>[5x]QELGNANFENFIGATEGFSEIAYQFTSHILTLGYAVMLAGLLYFILTIKNVDKKFQMSNILSAVVMVSAFLLLYAQAQNWTSSFTFNEEVGRYFLDPSGDLFNNGYRYLNWLIDVPMLLFQILFVVSLTTSKFSSVRNQFWFSGAMMIITGYIGQFYEVSNLTAFLVWGAISSAFFFH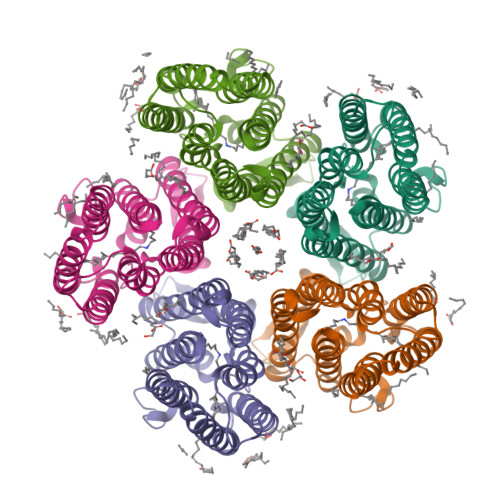ILWVMKKVINEGKEGISPAGQKILSNIWILFLISWTLYPGAYLMPYLTGVDGFLYSEDGVMARQLVYTIADVSSKVIYGVLLGNLAITLSKNKEL>[8x]MCFSPKIKTPKMDTNQIRAVEPAPLTQEVSSVEFGGSSDETDTEGTEVSGRKGLKVERDDSVAKSKASGNGSARMKSSIRKSAFGGKK;>[8x]MSKIESALQAAQPGLSRLRGGAGGMGYRAATTQAEQPRSSLLDTIGRFAKAGADMYTAKEQRARDLADERSNEIIRKLTPEQRREALNNGTLLYQDDPYAMEALRVKTGRNAAYLVDDDVMQKIKEGVFRTREEMEEYRHSRLQEGAKVYAEQFGIDPEDVDYQRGFNGDITERNISLYGAHDNFLSQQAQKGAIMNSRVELNGVLQDPDMLRRPDSADFFEKYIDNGLVTGAIPSDAQATQLISQAFSDASSRAGGADFLMRVGDKKVTLNGATTTYRELIGEEQWNALMVTAQRSQFETDAKLNEQYRLKINSALNQEDPRTAWEMLQGIKAELDKVQPDEQMTPQREWLISAQEQVQNQMNAWTKAQAKALDDSMKSMNKLDVIDKQFQKRINGEWVSTDFKDMPVNENTGEFKHSDMVNYANKKLAEIDSMDIPDGAKDAMKLKYLQADSKDGAFRTAIGTMVTDAGQEWSAAVINGKLPERTPAMDALRRIRNADPQLIAALYPDQAELFLTMDMMDKQGIDPQVILDADRLTVKRSKEQRFEDDKAFESALNASKAPEIARMPASLRESARKIYDSVKYRSGNESMAMEQMTKFLKESTYTFTGDDVDGDTV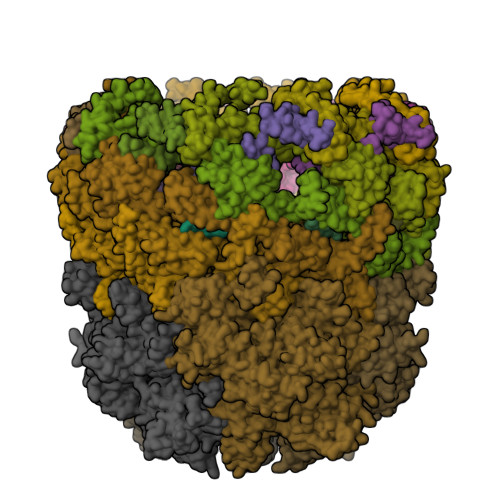GVIPKNMMQVNSDPKSWEQGRDILEEARKGIIASNPWITNKQLTMYSQGDSIYLMDTTGQVRVRYDKELLSKVWSENQKKLEEKAREKALADVNKRAPIVAATKAREAAAKRVREKRKQTPKFIYGRKE;>[4x]MDKYDKNVPSDYDGLFQKAADANGVSYDLLRKVAWTESRFVPTAKSKTGPLGMMQFTKATAKALGLRVTDGPDDDRLNPELAINAAAKQLAGLVGKFDGDELKAALAYNQGEGRLGNPQLEAYSKGDFASISEEGRNYMRNLLDVAKSPMAGQLETFGGITPKGKGIPAEVGLAGIGHKQKVTQELPESTSFDVKGIEQEATAKPFAKDFWETHGETLDEYNSRSTFFGFKNAAEAELSNSVAGMAFRAGRLDNGFDVFKDTITPTRWNSHIWTPEELEKIRTEVKNPAYINVVTGGSPENLDDLIKLANENFENDSRAAEAGLGAKLSAGIIGAGVDPLSYVPMVGVTGKGFKLINKALVVGAESAALNVASEGLRTSVAGGDADYAGAALGGFVFGAGMSAISDAVAAGLKRSKPEAEFDNEFIGPMMRLEARETARNANSADLSRMNTENMKFEGEHNGVPYEDLPTERGAVVLHDGSVLSASNPINPKTLKEFSEVDPEKAARGIKLAGFTEIGLKTLGSDDADIRRVAIDLVRSPTGMQSGASGKFGATASDIHERLHGTDQRTYNDLYKAMSDAMKDPEFSTGGAKMSREETRYTIYRRAALAIERPELQKALTPSERIVMDIIKRHFDTKRELMENPAIFGNTKAVSIFPESRHKGTYVPHVYDRHAKALMIQRYGAEGLQEGIARSWMNSYVSRPEVKARVDEMLKELHGVKEVTPEMVEKYAMDKAYGISHSDQFTNSSIIEENIEGLVGIENNSFLEARNLFDSDLSITMPDGQQFSVNDLRDFDMFRIMPAYDRRVNGDIAIMGSTGKTTKELKDEILALKAKAEGDGKKTGEVHALMDTVKILTGRARRNQDTVWETSLRAINDLGFFAKNAYMGAQNITEIAGMIVTGNVRALGHGIPILRDTLYKSKPVSAKELKELHASLFGKEVDQLIRPKRADIVQRLREATDTGPAVANIVGTLKYSTQELAARSPWTKLLNGTTNYLLDAARQGMLGDVISATLTGKTTRWEKEGFLRGASVTPEQMAGIKSLIKEHMVRGEDGKFTVKDKQAFSMDPRAMDLWRLADKVADEAMLRPHKVSLQDSHAFGALGKMVMQFKSFTIKSLNSKFLRTFYDGYKNNRAIDAALSIITSMGLAGGFYAMAAHVKAYALPKEKRKEYLERALDPTMIAHAALSRSSQLGAPLAMVDLVGGVLGFESSKMARSTILPKDTVKERDPNKPYTSREVMGAMGSNLLEQMPSAGFVANVGATLMNAAGVVNSPNKATEQDFMTGLMNSTKELVPNDPLTQQLVLKIYEANGVNLRERRK;>[8x]MCWAAAIPIAISGAQAISGQNAQAKMIAAQTAAGRRQAMEIMRQTNIQNADLSLQARSKLEEASAELTSQNMQKVQAIGSIRAAIGESMLEGSSMDRIKRVTEGQFIREANMVTENYRRDYQAIFAQQLGGTQSAASQIDEIYKSEQKQKSKLQMVLDPLAIMGSSAASAYASGAFDSKSTTKAPIVAAKGTKTGR>MVTVFGILNLTEDSFFDESRRLDPAGAVTAAIEMLRVGSDVVDVGPAASHPDARPVSPADEIRRIAPLLDALSDQMHRVSIDSFQPETQRYALKRGVGYLNDIQGFPDPALYPDIAEADCRLVVMHSAQRDGIATRTGHLRPEDALDEIVRFFEARVSALRRSGVAADRLILDPGMGFFLSPAPETSLHVLSNLQKLKSALGLPLLVSVSRKSFLGATVGLPVKDLGPASLAAELHAIGNGADYVRTHAPGDLRSAITFSETLAKFRSRDARDRGLDHA[2x]

The sulfonamides (sulfas) are the oldest class of antibacterial drugs and inhibit the bacterial dihydropteroate synthase (DHPS, encoded by folP), through chemical mimicry of its co-substrate p-aminobenzoic acid (pABA). Resistance to sulfa drugs is mediated either by mutations in folP or acquisition of sul genes, which code for sulfa-insensitive, divergent DHPS enzymes. DHPS catalyzes the condensation of para-aminobenzoic acid (pABA) and 6-hydroxymethyl-7,8-dihydropterin pyrophosphate (DHPP), producing 7,8-dihydropteroic acid (7,8-DHP); this compound is further transformed, ultimately leading to tetrahydrofolate, an essential precursor for DNA and RNA synthesis. All three Sul enzymes adopted the (ɑ/β)8 TIM barrel fold also shared by DHPS.

We determined the crystal structure of Sul1 in a ligand-bound state, and the Sul2 and Sul3 enzymes in both apo and ligand-bound forms to resolutions between 1.74 to 2.8 Å. We identified electron density in the active site of Sul1 corresponding only to a pterin ring which we modeled as 6-hydroxymethylpterin (6-HMP). The 6-HMP molecule formed hydrogen bonds with the Sul1 residues Asn101, Asp173 and Lys212. Additionally, the plane of the pterin ring formed van der Waals interactions with Phe179 and Ile103. We noticed that the Phe residue that is conserved across Sul enzymes (Phe178 in Sul1, Phe179 in Sul2 and Phe177 in Sul3) and localized to the active site adopted different rotamer conformations depending on ligand binding.> QAVLDVLKFYDSN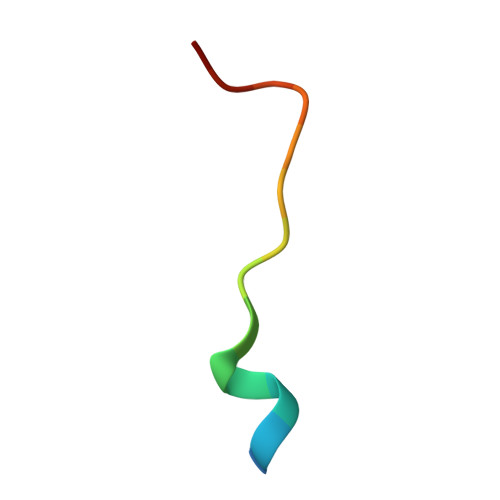TVK>MDTTTATTARTDTLLQLDNQLSFALYSANLAMHKLYRGLLKALDLTYPQYLVMLVLWETDERSVSEIGERLYLDSATLTPLLKRLQAAGLVTRTRAASDERQVIIALTETGRA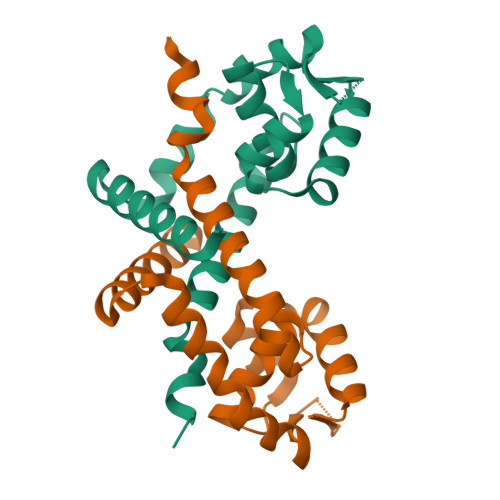LRSKAGAVPEQVFCASACSLDELRQLKQELEKLRSSLGAG[2x]> MLYRGLRMAARAAPKFAVLNTHAALR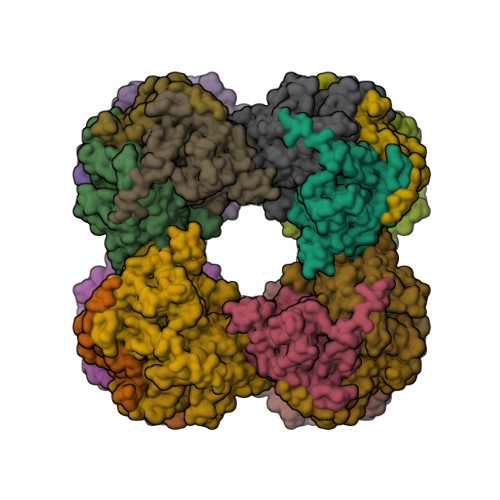QLPLQFQHVRTYADKIIKVPQMAESITEGTLKQWNKAVGDYVEADEEIATIETDKIDVAVNAPEAGVIKEFFVNEEDTVLVGQDLVRLEVGGEKPAEAAKEQPKAAAPEPKVEEKKVPEAPAPEPSKTAAPAPAPPKQEAPASPKPASKPAETPAVTLGNREERRVKMNRMRLRIAERLKQSQNTAASLTTFNEVDMSALIEFRNKYKDEVLKKTGVKLGFMSAFSRAVVLAIRDLPVVNASIEGPNGGDTIVYRDYVDISVAVATEKGLVTPVVRNAETMDLITIEKTIAELGKKARDGKLTIEDMAGGTFTISNGGVFGSLMGTPIINLPQSAVLGLHAIKERPVAVNGKVEIRPMMYLALTYDHRLLDGREAVQFLVKVKEYIEDPRKMLL>[2x]RDGRTFVVREKQVESAYVTSFVLVPADGGAVLDYQPGQYIGIEVTPEGSDYREIRQYSLSHASNGREYRISVKREGVGSDNPGLVSHYLHNNVKVGD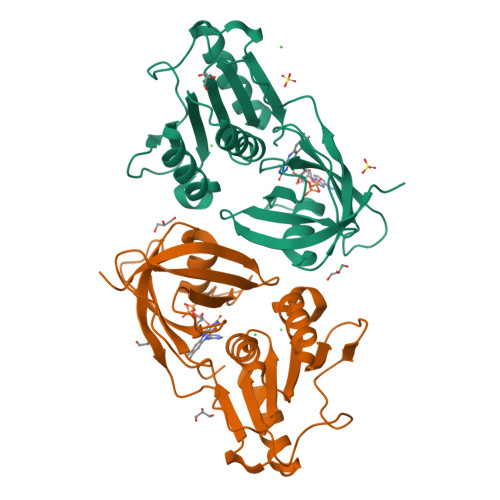SVKLYAPAGDFFYVERERPVVLISAGVGATPMQAILHTLAKQNKSGVTYLYACNSAKEHTFAQETAQLIAQQGWMQQVWYRDESADDVLQGEMQLAELILPIEDGDFYLCGPIGFMQYVVKQLLALGVDKARIHYEVFGPHAQLAA> MPSELTPEERSELKNSIAEFHTYQLDPGSCSSLHAQRIHAPPELVWSIVRRFDKPQTHRHFIKSCSVEQNFEMRVGCTRDIIVISGLPANTSTERLDILDDERRVTGASIIGGEHRLTNYKGVTTVHRFEKENRIWTVVLESYVVDMPEGNSEDDTRIVVDDV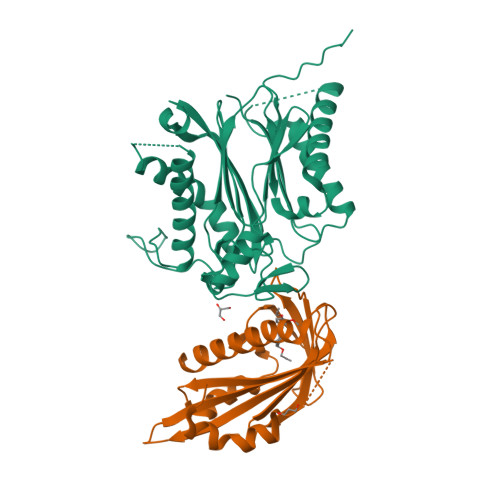VKLNLQKLATVAEAMARN;> RSVYELDCIPLWGTVSIQGNASEMEAAFAVSPHFLKLPIKMLMGDHEGMSPSLTHLTGHFFGVYDGHGGHKVADYCRDRLHFALAEEIERIKDELCKRNTGEGRQVQWDKVFTSCFLTVDGEIEGKIGRAVVGSSDKVLEAVADETVGSTAVVALVCSSHIVVSNCGDSRAVLFRGKEAMPLSVDHKPDREDEYARIENAGGKVIQWQGARVFGRLAMSRSIGDRYLKPYVIPEPEVTFMPRSREDECLILASDGLWDVMNNQEVCEIARRRILMWHKKNGAPPLAERGKGIDPACQAAADYLSMLALQKGSKDNISIIVIDLKAQRKFKTAT> MAHHHHHHMDAATTRAGLTDLKFRLVRESFADAVSWVAKNLPTRPAVPVLSGVLLTGSDEGLTISGFDYEVSAEVRVPAEIASPGTVLVSGRLLSDITRALPNKPVDFYVDGNRVALTCGNARFSLPTMAVEDYPTLPTLPEDTGTLPAELFSEAIGQVAIAAGRDDTLPMLTGIRVEISGEKVVLAATDRFRLAVRELTWNALSPDIEAAVLVPAKTLGEAAKANTDGSEVRLSLGAGMGVGKDGLLGISGDGKRSTTRLLDAEFPKFRQLLPAEHTAVAS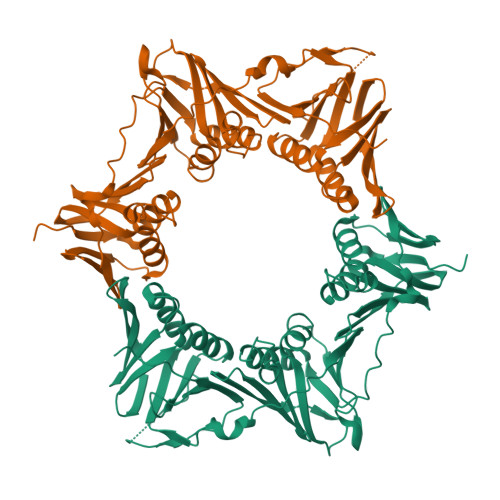ADVAELTEAIKLVALVADRGAQVRMEFADGMLRLSAGADDVGRAEEDIAVEFAGQPLTIAFNPTYLIDGLASLHSERVSFGFTTPGKPALLRPASAEDRIVSGPGDQGPFAAVPTDYVYLLMPVRLPG> SKGKSSGKK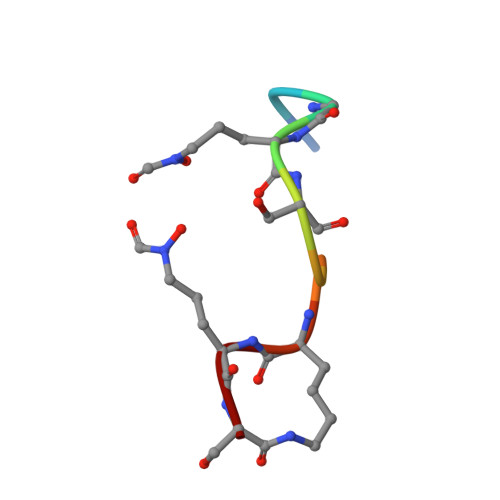S>ADPVYSFSQQPQDQVVVSGQPVTLLCAIPEYDGFVLWIKDGLALGVGRDLSSYPQYLVVGNHLSGEHHLKILRAELQDDAVYECQAIQAAIRS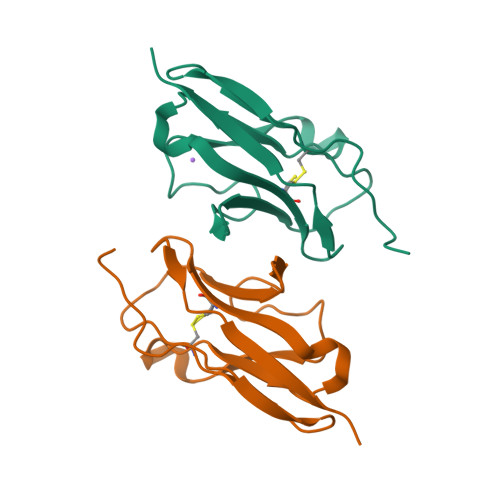RPARLTVLVPHHHHHH[8x]Kynurenine-3-monooxygenase (KMO) is a class A flavoprotein monooxygenase (FPMO) which catalyses the hydroxylation of L-kynurenine (L-Kyn) to 3-hydroxykynurenine (3-HK), using NADPH as a co-substrate. It lies at a key branch point of the kynurenine pathway and its expression is largely restricted to the liver, kidney, some monocytic cells, and to a lesser extent in the microglia within the brain. We therefore turned our attention to the homologous bacterial P. fluorescens enzyme, Pf-KMO, which shares 34% sequence identity with the human enzyme, but lacks the transmembrane region and had been previously extensively characterized by Crozier-Reabe et al.. The KMO monomer consists of three domains: the α+β FAD-binding domain, an α+β domain containing a six-stranded, mostly antiparallel, β-sheet and a C-terminal four-helix bundle domain.

Further rounds of improvement were successful in delivering a high resolution-diffracting monoclinic crystal form with two holoenzyme molecules in the asymmetric unit that was amenable to ligand soaking studies.

>[2x]MTATDNARQVTIIGAGLAGTLVARLLARNGWQVNLFERRPDPRIETGARGRSINLALAERGAHALRLAGLEREVLAEAVMMRGRMVHVPGTPPNLQPYGRDDSEVIWSINRDRLNRILLDGAEAAGASIHFNLGLDSVDFARQRLTLSNVSGERLEKRFHLLIGADGCNSAVRQAMASVVDLGEHLETQPHGYKELQITPEASAQFNLEPNALHIWPHGDYMCIALPNLDRSFTVTLFLHHQSPAAQPASPSFAQLVDGHAARRFFQRQFPDLSPMLDSLEQDFEHHPTGKLATLRLTTWHVGGQAVLLGDAAHPMVPFHGQGMNCALEDAVALAEHLQSAADNASALAAFTAQRQPDALAIQAMALENYVEMSSKVASPTYLLERELGQIMAQRQPTRFIPRYSMVTFSRLPYAQAMARGQIQEQLLKFAVANHSDLTSINLDAVEHEVTRCLPPLSHLS> MLRRLVPRVMMAPMGGATALCTSRGYNMLVFRDPKRRPQLSEEERAKVVVNQAEWPEEFKDFDPDDPYKNSPEIIKGMSSWNLFLWGVECAFIYQFY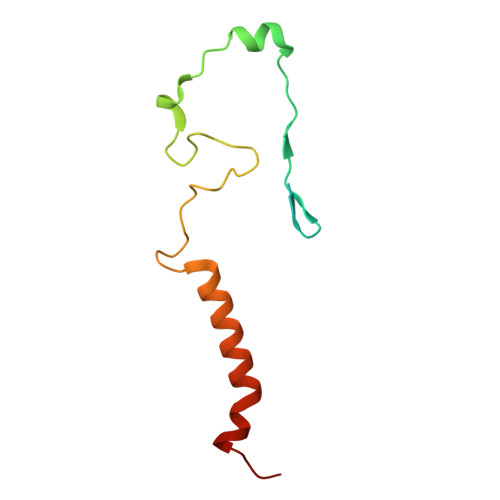ELVFPKSI> AHHHHHHPGGPGSDELDLNLAYPISPWKFKLFCGPPNTTDDSFLSPAGAPNNASALKGASEAIVEAKFNSSGIYVPELSKTVFHCCFGNEQGQNCSALTDNTEGKTLASVVKASVFRQLGVNWDIECWMKGDLTLFICHMEPLPKNPFKNYDSKVHLLYDLPEVIDDSPLPPLKDSFQTVQCNCSLRGCECHVPVPRAKLNYALLMYLEITSAGVSFQSPLMSLQPMLVVKPDPPLGLHMEVTDDGNLKISWDSQTMAPFPLQYQVKYLENSTIVREAAEIVSATSLLVDSVLPGSSYEVQVRSKRLDGSGVWSDWSSPQVFTTQDVVYFPPKILTSVGSNASFHCIYKNENQIISSKQIVWWRNLAEKIPEIQYSIVSDRVSKVTFSNLKATRPRGKFTYDAVYCCNEQACHHRYAELYVIDVNINISCETDGYLTKMTCRWSPSTIQSLVGSTVQLRYHRRSLYCPDSPSIHPTSEPKNCVLQRDGFYECVFQPIFLLSGYTMWIRINHSLGSLDSPPTCVLPDSVVKPLPPSNVKAEITVNTGLLKVSWEKPVFPENNLQFQIRYGLSGKEIQWKTHEVFDAKSKSASLLVSDLCAVYVVQVRCRRLDGLGYWSNWSSPAYTLVMDVKVPMRGPEFWRKMDGDVTKKERNVTLLWKPLTKNDSLCSVRRYVVKHRTAHNGTWSEDVGNRTNLTFLWTEPAHTVTVLAVNSLGASLVNFNLTFSWPMSKVSAVESLSAYPLSSSCVILSWTLSPDDYSLLYLVIEWKILNEDDGMKWLRIPSNVK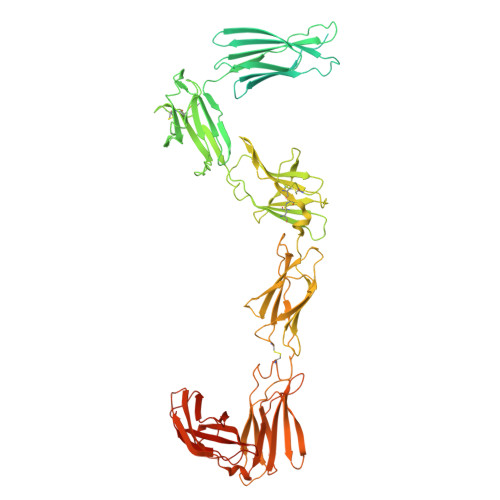KFYIHDNFIPIEKYQFSLYPVFMEGVGKPKIINGFTKDAIDKQQNDAG>GSIAPYLVKIIDPDYEKNERTRIKAQENLRRIRRKQIAEKGDNEDGTDDPSRRRKIDDLVLNEYENQVALEVVAPEDIPVGFNDIGGLDDIIEELKETIIYPLTMPHLYKHGGALLAAPSGVLLYGPPGCGKTMLAKAVAHESGASFINLHISTLTEKWYGDSNKIVRAVFSLAKKLQPSIIFIDEIDAVLGTRRSGEHEASGMVKAEFMTLWDGLTSTNASGVPNRIVVLGATNRINDIDEAILRRMPKQFPVPLPGLEQRRRILELVLRGTKRDPDFDLDYIARVTAGMSGSDIKETCRDAAMAPMREYIRQHRASGKPLSEINPDDVRGIRTEDFFGRRGGKILSEIPPRQTG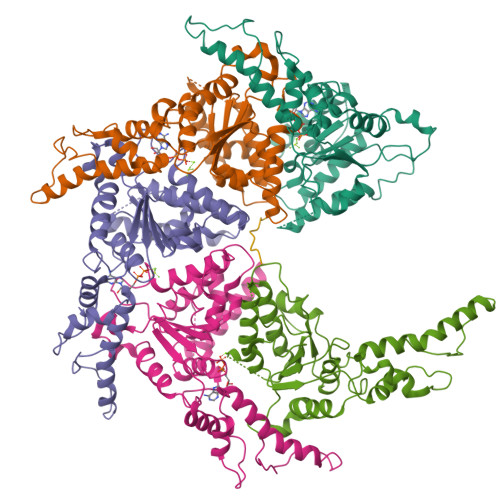YVVQSKNSSEGGYEEVEDDDEQGTAST[5x]>[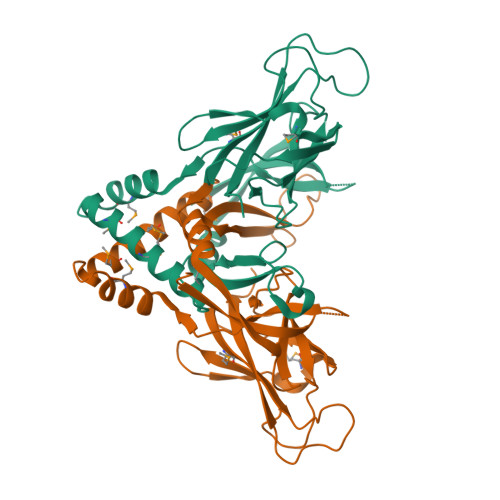4x]GAKNVLKAWLVDNTVTTDDKTDKIFQLETTRSIDKEIILDRMVAKNPGVRRETMALGIELMEEVVAEALMNGESVNTGLFRGVAQFRGVAKQNAWDAATNSIYVSLTQGKALREAIKDTRVDVLGERPTKFYIGSGQDATTRATDFSATAGRNFTLFGKNLTVAGTDPSVGVTLASAATGTVTKIDNDMIVLNEPSRLIILLPASLEDGEYMLTVTTQYRGGGGALLKTPRSTSHTIYIGGAPETGGSTGPPGDSDGDLNENPLG> MYTAIPQSGSPFPGSVQDPGLHVWRVEKLKPVPVAQENQGVFFSGDSYLVLHNGPEEVSHLHLWIGQQSSRDEQGACAVLAVQLDDYLGGRPVQHREVQGNESDLFMSYFPRGLKYQEGGVESGFKHVVPNEV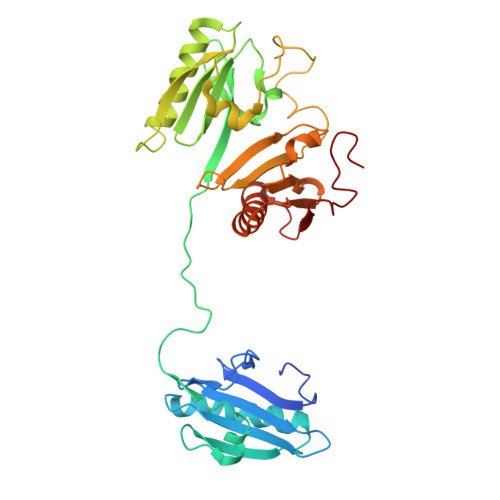VVQRLYQVKGKKNIRATERALNWDSFNTGDCFILDLGQNIFAWCGGKSNILERNKARDLALAIRDSERQGKAQVEIVTDGEEPAEMIQVLGPKPALKEGNPEEDLTADKANAQAAALYKVSDATGQMNLTKVADSSPFALELLISDDCFVLDNGLCGKIYIWKGRKANEKERQAALQVAEGFISRMQYAPNTQVEILPQGRESPIFKQFFKDWK> MYAPAAEDEHTITNWSGTHAVRPKRFFQPESVEELEKIVKEAHEKGQKIRPVGSGLSPNGLAFSEDGMVSLALMDKVLHVDKEKKQVTVQAGARVQQVVDALRPHGLTLQNFASISEQQIGGFIQVGAHGTGARIPPVDEQVVSMKLVTPAKGTIELSEEKDPELFRLARCGLGALGVVTEVTLQCVPRHKLLEHTFVATMKEVKKNHEKLLRENKHVRYMWIPYTDTVVVVTCNPLPEGKKAPKVKPQYSEDEKLQPLRNLLREAAPPARAPEVAAPSSSETSPEVSGLSFTELRDALLAVDPLDTEWVKRVNQAEAEFWKRSEGYRVGWSDEILGFDCGGQQWVSEVAFPAGTLEKPSAADLEYMEELMRLINKEGIPAPAPIEQRWTAGSSSPMSPAYSPSPDSVFSWVGIIMYLPTEDEEQRKAITEAFRQYRKLCETRLWDKYGAAEHWAKIEVPEDPEELEALRERLRKRYPGVDKFNKARRELDPKNILSNDMIDSLFPAAESA

In photosynthetic organisms, L-ascorbic acid is produced in the Smirnoff-Wheeler pathway by the multi-step conversion of D-mannose-6-phosphate to L-galactono-1,4-lactone, the substrate for the final biosynthetic enzyme, L-galactono-1,4-lactone dehydrogenase (GalDH) [EC 1.3.2.3]9,15. GULO, ALO, and GalDH are generally named aldonolactone oxidoreductases and form a group of sequence-related flavoenzymes belonging to the vanillyl-alcohol oxidase family. They oxidize the C2 carbon atom of their monosaccharide substrates and thereby generate the characteristic, redox-reactive C2-C3 double bond of L-ascorbic acid and its analogs. GalDH is a dehydrogenase that reacts poorly with oxygen.

To elucidate the structural features of GalDH and how it interacts with its substrate, we determined the crystal structures of the viridiplantae ancestor without (1.9 Å resolution) and with L-galactono-1,4-lactone (2.1 Å resolution). Soaking in a substrate-containing solution led to the bleaching of the crystals and the resulting electron density clearly indicated the presence of the bound substrate. We, therefore, conclude that the crystals accumulate the substrate-bound reduced state, outlining the structure of the Michaelis complex. Upon substrate binding, the movement of a gating loop (residues 337-344) constricts the access to the active site, creating the catalytic cavity. L-galactono-1,4-lactone adopts a pro-catalytic conformation with its C2 carbon at 3.1 Å distance from the isoalloxazine ring and C2 hydrogen predicted to point towards the flavin N5 position. The surrounding side chains establish a hydrogen bond network with the ligand hydroxyl groups. These interactions are enforced by the closure of the gating loop with two of its residues, Cys340 and Gln344, moving closer to the sugar to interact with its 1 and 5 oxygens. Arg388 and Lys456 critically position their positively charged side chains in contact with the substrate O2 atom, confirming previous hypotheses about the importance of Arg388 for enzyme activity. In particular, these residues may promote the binding of the alkoxide anion of the substrate, which in turn facilitates hydride transfer from the C2 position to the flavin N5, leading to substrate oxidation. The resulting 1,2-diketo product will then spontaneously tautomerize to the more stable enediol form of vitamin C32.>MTIMEVQVVSKKMVKPSVPTPDHHKTCKLTAFDQIAPPDQVPIIYFYNSSNIHNIREQLVKSLSETLTKFYPLAGRFVQDGFYVDCNDEGVLYVEAEVNIPLNEFIGQAKKNIQLINDLVPKKNFKDIHSYENPIVGLQMSYFKCGGLAICMYLSHVVADGYTAAAFTKEWSNTTNGIINGDQLVSSSPINFELATLVPARDLSTVIKPAVMPPSKIKETKVVTRRFLFDENAISAFKDHVIKSESVNRPTRVEVVTSVLWKALINQSK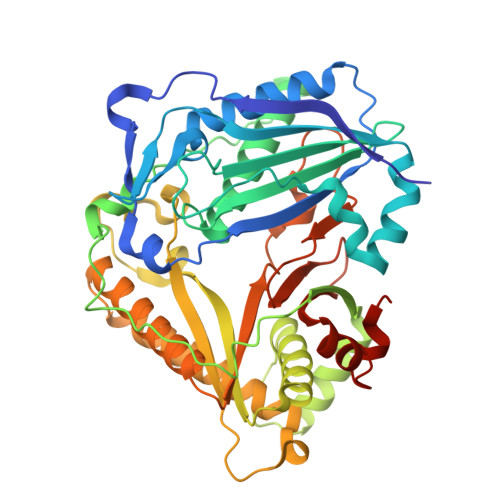LPSSTLYFHLNFRGKTGINTPPLDNHFSLCGNFYTQVPTRFRGGNQTKQDLELHELVKLLRGKLRNTLKNCSEINTADGLFLEAASNFNIIQEDLEDEQVDVRIFTTLCRMPLYETEFGWGKPEWVTIPEMHLEIVFLLDTKCGTGIEALVSMDEADMLQFELDPTISAFASLEHHHHHH[2x]> MTINKLSLTDELLNNFGGSTEVDSVLKNIDFDVSDDASKVLSLSTDYNARNLMALSLVLANNDNINNYNQKYIQKVITVIDKLIDLQVNSIISNDEFRALEQEWLKVQEVCQEDYDNVEV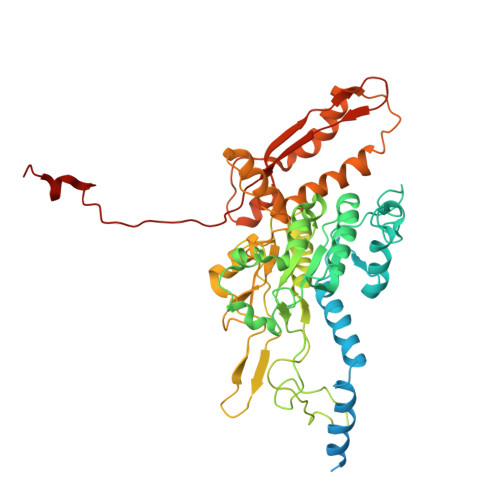SILDVKKEELQYDFERNLYDISSSDFFKKVYVSEFDQYGGEPYGAILGLYNFENTTNDIIWLTGMGMVAKNSHAPFIASIDKSFFGVKDLSEITHIKSFEALLEHPRYKEWNDFRNLDVAAYIGLTVGDFMLRQPYNPENNPVQYKLMEGFNEFVDYDKNESYLWGPASIHLVKNMMRSYDKTRWFQYIRGVESGGYVKNLVACVYDNKGILETKSPLNVLFADYMELSLANIGLIPFVSEKGTSNACFFSVNSAKKVEEFVDGFDSANSRLIANLSYTMCISRISHYIKCVIRDKIGSIVDVESIQKILSDWISEFVTTVYQPTPLEMARYPFRNVSIEVKTIPGKPGWYSCKINVIPHIQFEGMNTTMTIDTRLEPELFGTNNN>[2x]MSYQSTIVPVELHSFEDAQVIGGA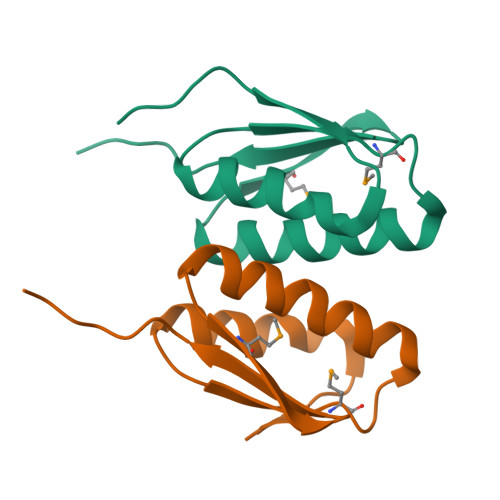FRDGDAVVFDMSLLSREEARRIVDFAAGLCFALHGKMQKIDSVTFAVVPELSNISLEHHHHHH>GPGLKQKIVIKVAMEGNNCRSKAMALVASTGGVDSVALVGDLRDKIEVVGYGIDPIKLISALRKKVGDAELLQVS[2x];> METGNKYIEKRAIDLSRERDPNFFDHPGIPVPECFWFMFKNNVRQDAGTCYSSWKMDMKVGPNWVHIKSDD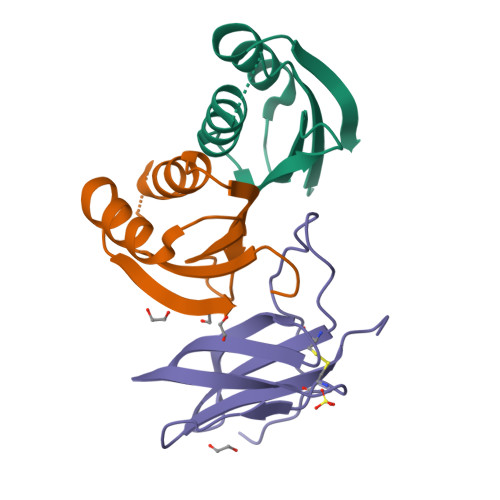NCNLSGDFPPGWIVLGKKRPGF> GSHMLQSTPQNLVSNAPI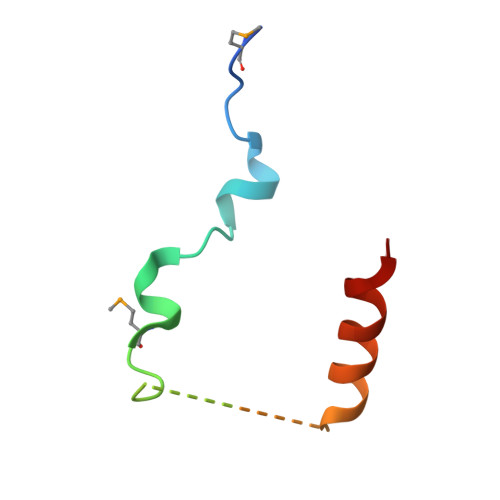AETAMGIAEPIGAGSEFHGNPDDDLQARLNTLKKQT>SNAQQSQAFECTLVTSIETGAVINQQGACDQRVAPASTFKVPLALIGYDAGILLDDKTPAWDWKPGTEARAQDRKTVDPTIWEQDSVLWYSRELTRRLGPEKFAAYVKRLGYGNADVSGEPGKNNGLTHSWLGASLTVSPVEQVGFIRRLLAGNLPVSRDAQAKTRAIVPVFYAPESWSVHGKTGTGFMRDEKGNPDR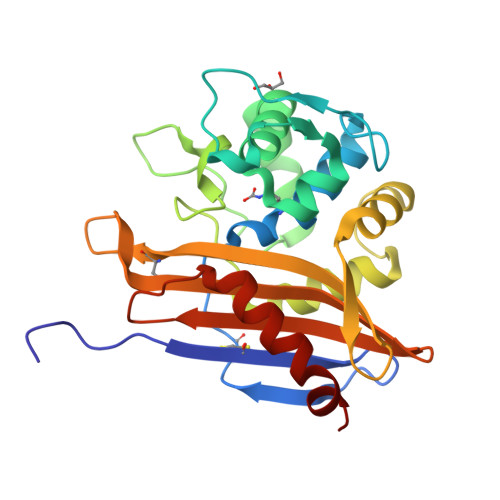SRPFGWFVGWAEREGQHIVFARLRVADKPSSEPLGPAVRDAFLRDIARLAVHR[4x]Named for their conserved Walker B motif consisting of adjacent aspartate-glutamate-alanine-aspartate (D-E-A-D) residues, DEAD-box proteins are required for all stages of RNA metabolism including transcription, processing and splicing, export, translation and decay. DEAD-box proteins bind nucleotides via the canonical Walker A and B motifs and the family-specific Q-motif that recognizes the adenine of ATP and makes the DEAD-box proteins ATP-specific. ATP binding and hydrolysis drive non-processive unwinding of RNA substrates by local strand separation. In this work, we describe a chemical genetic strategy for the specific inactivation of individual DEAD-box proteins with small molecule inhibitors using covalent complementarity.

To better understand the binding of AMP-acrylates to ES DEAD-box proteins, we solved the crystal structure of DDX3 (132–607) S228C bound to AMP-acrylamide to 3.0 Å. The overall protein structure is highly similar to the previously published structure of DDX3 bound to AMP, with a root mean squared deviation of 1.265 Å, as expected from its similar thermal stability. AMP-acrylamide can be fit unambiguously to its density and clearly binds cysteine-228 through a covalent bond. The adenine of AMP-acrylamide maintains several hydrogen-bonding interactions with the Q-motif of DDX3 including interactions with glutamine-207 and the backbone of arginine-202, as well as pi-stacking with tyrosine-200. The covalent linkage significantly re-orders the P-loop into a conformation that to our knowledge has not previously been observed in nucleotide-bound structures of DEAD-box proteins. This results in a 9.4 Å shift in the side chain of T226 as compared to AMP-bound DDX3. In addition, the phosphoramidate of AMP-acrylamide is also displaced more than 3 Å out of the phosphate-binding pocket as compared to the phosphate of AMP so that only the 5′-oxygen hydrogen bonds with the P-loop backbone, whereas the phosphate of AMP typically makes numerous electrostatic interactions. The significant flattening of the P-loop observed in this structure is likely due to the torsion placed on this flexible loop by the tethered small molecule as it moves to maintain hydrogen bonds within the Q-motif. Interestingly, this distortion of the P-loop breaks the electrostatic interactions between the phosphate and the P-loop backbone, which are typically thought to drive nucleotide affinity. Nonetheless, we expect the reordering of the P-loop observed upon binding of this compound to strongly antagonize the closed (active) conformation of DDX3.

> GSFTDEDDWSKPLPPSERLEQELFSGGNTGINFEKYDDIPVEATGNNCPPHIESFSDVEMGEIIMGNIELTRYTRPTPVQKHAIPIIKEKRDLMACAQTGCGKTAAFLLPILSQIYSDGPGEALRAMKENGRYGRRKQYPISLVLAPTRELAVQIYEEARKFSYRSRVRPCVVYGGADIGQQIRDLERGCHLLVATPGRLVDMMERGKIGLDFCKYLVLDEADRMLDMGFEPQIRRIVEQDTMPPKGVRHTMMFSATFPKEIQMLARDFLDEYIFLAVGRVGSTSENITQKVVWVEESDKRSFLLDLLNATGKDSLTLVFVETKKGADSLEDFLYHEGYACTSIHGDRSQRDREEALHQFRSGKSPILVATAVAARGLDISNVKHVINFDLPSDIEEYVHRIGRTGRVGNLGLATSFFNERNINITKDLLDLLVEAKQEVPSWLENMAYEHHYKGSSRGRSKSSRFSGGFGARDYRQSSG>[2x]MSRGH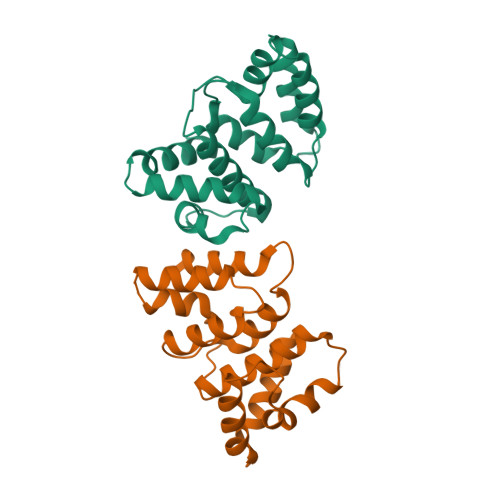HHHHHGSMSPGERFLDWLKRLQGQKAWTAARAAFRRSLAFPPGAYPRAMPYVEPFLAKGDWRQEEREAHYLVAALYALKDGDHQVGRTLARALWEKAQGSASVEKRFLALLEADRDQIAFRLRQAVALVEGGIDFARLLDDLLRWFSPERHVQARWAREYYGA>MSYTPGQPVTAVVQRVEIHKLRQGENLILGFSIGGGIDQDPSQNPFSEDKTDKGIYVTRVSEGGPAEIAGLQIGDKIMQVNGWDMTMVTHDQARKRLTKRSEEVVRLLVTRQSLQKAVQQSMLS[2x];>[2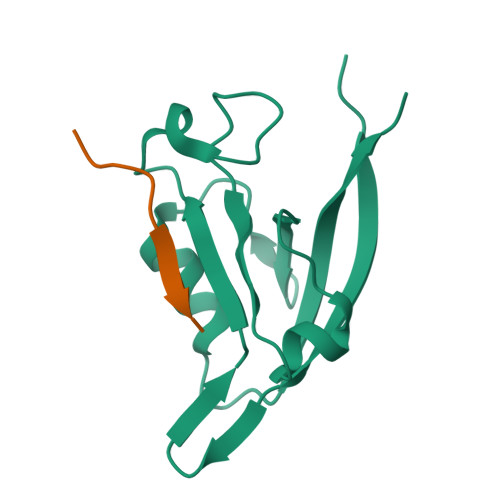x]NQLAWFDTDL NA, which is a sialidase, catalyzes hydrolysis of terminally linked sialic acid and functions as the receptor-destroying element of influenza A and B viruses. Additionally, influenza A NA is further classified into two groups: group 1 (N1, N4, N5 and N8) and group 2 (N2, N3, N6, N7 and N9), based upon primary sequence. Group 1 NAs contain a 150-cavity (formed by amino acids 147–151 of the 150-loop) in their active site, whereas group 2 NAs lack this cavity. NA inhibition assays were carried out and complex crystal structures were solved for laninamivir, laninamivir octanoate, zanamivir and oseltamivir in order to elucidate the structural basis of their inhibition.

To determine the functional and structural basis of NA inhibition and binding by laninamivir and its prodrug, we first expressed and purified a new group 2 member from the 1957 pandemic H2N2 virus, p57N2, using similar methods. Like the available group 2 A/TOKYO/3/1967 (H2N2) N2 and A/Memphis/31/98 (H3N2) N2 structures, p57N2 also contains a 150-cavity deficient active site with a salt bridge between Asp147 and His150, confirming the presence of a stable, closed 150-loop. To determine the structural basis of the inhibition of laninamivir relative to zanamivir, we solved the very first complex structures of laninamivir with p57N2, p09N1 and N5 at resolutions of 1.8 Å, 1.8 Å and 1.6 Å, respectively; and the complex structures of zanamivir with p57N2, p09N1 and N5 at 1.9 Å, 1.9 Å and 1.6 Å, respectively. Like zanamivir, the binding mode of laninamivir to all 3 NAs is highly similar to that of the NA transition state analogue, Neu5Ac2en. In all of the zanamivir and laninamivir structures, the 4-guanidino group is buried deep beneath the 150-loop where it forms many key hydrogen bonds with Glu119, the Trp178 peptide carbonyl, Glu227, and the Asp151 side chain and peptide carbonyl. Although this laninamivir 7-methoxy group is oriented away from its own ring oxygen and is pointed toward the hydrophobic Ile222 side chain, its distance is relative far at over 5 Å. On the other hand, the carboxylate-Arg292 interactions are further in zanamivir than laninamivir in every NA complex. Laninamivir inhibition was best for group 1 N5, followed by atypical group 1 p09N1 and worst for group 2 p57N2. Laninamivir was in a similar range with zanamivir for N5, p09N1 and p57N2 with IC50 values of 0.90 nM, 1.83 nM and 3.12 nM, respectively. Group 2 p57N2 contains an Asp147-His150 salt bridge, limiting the flexibility of its closed 150-loop and inhibition of p57N2 by laninamivir was the lowest. p09N1 is an atypical group 1 with no 150-cavity, but no Asp147-His150 salt bridge, and inhibition of p09N1 by laninamivir was better than p57N2.

>MNPNQKIITIGSVSLTIATVCFLMQIAILATTVTLHFKQHECDSPASNQVMPCEPIIIERNITEIVYLNNTTIEKEICPKVVEYRNWSKPQCQITGFAPFSKDNSIRLSAGGDIWVTREPYVSCDPGKCYQFALGQGTTLDNKHSNDTVHDRIPHRTLLMNELGVPFHLGTRQVCIAWSSSSCHDGKAWLHVCITGDDKNATASFIYDGRLVDSIGSWSQNILRTQESECVCINGTCTVVMTDGSASGRADTRILFIEEGKIVHISPLSGSAQHIEECSCYPRYPGVRCICRDNWKGSNRPVVDINMEDYSIDSSYVCSGLVGDTPRNDDSSSNSNCRNPNNERGTQGVKGWAFDNGNDLWMGRTISKESRSGYETFKVIGGWSTPNSKSQVNRQVIVDNNNWSGYSGIFSVEGKSCINRCFYVELIRGRPQETRVWWTSNSIVVFCGTSGTYGTGSWPDGANINFMPI[4x]>MGELVRTDSPNFLCSVLPTHWRCNKTLPIAFKVVAKGDVPDGTLVTVMAGNDENYSAELRNATAAMKNQVARFNDLRFVGRSGRGKSFTLTITVFTNPPQVATYHRAIKITVDGPREPRRHRQKLDDQTKPGSLSFSERLSELEQLRRTAMR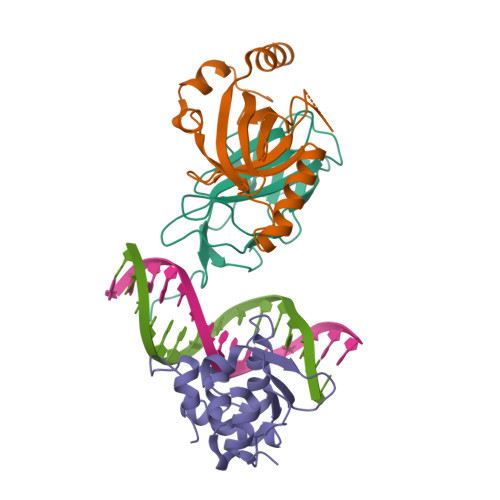VSPHHPAPTPNPRASLNHSTAFNPQPQSQMQDARQIQPSPPWSYDQSYQYLGS[2x];>[2x]MPRVVPDQRSKFENEEFFRKLSRECEIKYTGFRDRPHEERQTRFQNACRDGRSEIAFVATGTNLSLQFFPASWQGEQRQTPSREYVDLEREAGKVYLKAPMILNGVCVIWKGWIDLHRLDGMGCLEFDEERAQQEDALAQQA;>SLQRVPSYDSFDSEDYPAALPNHKPKGTFKDYVRDRADLNKDKPVIPAAALAGYTGSGPIQLWQFLLELLTDKSCQSFISWTGDGWEFKLSDPDEVARRWGKRKNKPKMNYEKLSRGLRYYYDKNIIHKTAGKRYVYRFVCDLQSLLGYTPEELHAMLDVKPDADE[2x]>MGPKLFKPSIDWSRAFPDSVYWVGKAWTISAICVLAILVLLRYLTPWGRQFWRITRAYFVGPNSVRVWLMLGVLLLSVVLAVRLNVLFSYQGNDMYTALQKAFEGIASGDGTVKRSGVRGFWMSIGVFSVMAVLHVTRVMADIYLTQRFIIAWRVWLTHHLTQDWLDGRAYYRDLFIDETIDNPDQRIQQDVDIFTAGAGGTPNAPSNGTASTLLFGAVQSIISVISFTAILWNLSGTLNIFGVSIPRAMFWTVLVYVFVATVISFIIGRPLIWLSFRNEKLNAAFRYALVRLRDAAEAVGFYRGERVEGTQLQRRFTPVIDNYRRYVRRSIAFNGWNLSVSQTIVPLPWVIQAPRLFAGQIDFGDVGQTATSFGNIHDSLSFFRNNYDAFASFRAAIIRLHGLVDANEKGRALPAVLTRPSDDESVELNDIEVRTPAGDRLIDPLDVRLDRGGSLVITGRSGAGKTTLLRSLAELWPYASGTLHRPGGENETMFLSQLPYVPLGTLRDVVCYPNSAAAIPDATLRDTLTKVALAPLCDRLDEERDWAKVLSPGEQQRVAFARILLTKPKAVFLDGSTSALDTGLEFALYQLLRSELPDCIVISVSHRPALERLHENQLELLGG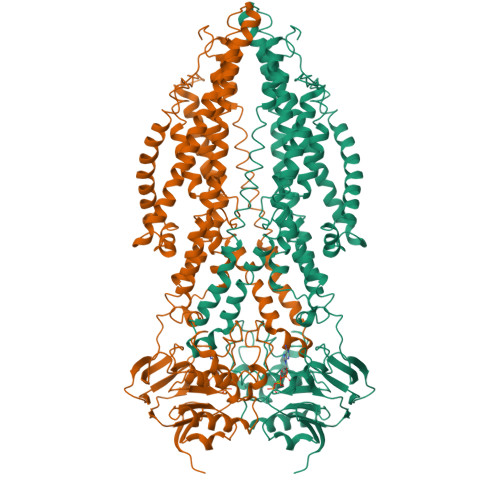GQWRLAPVEAAPAEVHHHHHHHH[2x]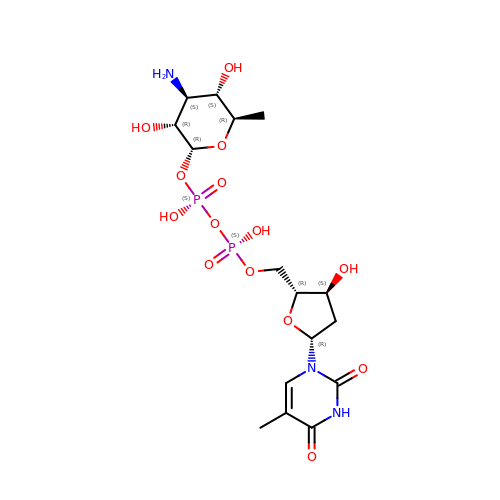[(3R,4S,5S,6R)-4-amino-3,5-dihydroxy-6-methyloxan-2-yl][hydroxy-[[(2R,3S,5R)-3-hydroxy-5-(5-methyl-2,4-dioxopyrimidin-1-yl)oxolan-2-yl]methoxy]phosphoryl] hydrogen phosphate | C16 H27 N3 O14 P2 | KVYJLJOGNUNRJK-HALQBZCBSA-N> APSPIIKFPGDVAPKTDKELAVQYLNTFYGCPKESCNLFVLKDTLKKMQKFFGLPQTGDLDQNTIETMRKPRCGNPDVANYNFFPRKPKWDKNQITYRIIGYTPDLDPETVDDAFARAFQVWSDVTPLRFSRIHDGEADIMINFGRWEHGDGYPFDGKDGLLAHAFAPGTGVGGDSHFDDDELWTLGEGQVVRVKYGNADGEYCKFPFLFNGKEYNSCTDTGRSDGFLWCSTTYNFEKDGKYGFCPHEALFTMGGNAEGQPCKFPFRFQGTSYDSCTTEGRTDGYRWCGTTEDYDRDKKYGFCPETAMSTVGGNSEGAPCVFPFTFLGNKYESCTSAGRSDGKMWCATTANYDDDRKWGFCPDQGYSLFLVAAHAFGHAMGLEHSQDPGALMAPIYTYTKNFRLSQDDIKGIQELYGASPDIDLGTGPTPTLGPVTPEICKQDIVFDGIAQIRGEIFFFKDRFIWRTVTPRDKPMGPLLVATFWPELPEKIDAVYEAPQEEKAVFFAGNEYWIYSASTLERGYPKPLTSLGLPPDVQRVDAAFNWSKNKKTYIFAGDKFWRYNEVKKKMDPGFPKLIADAWNAIPDNLDAVVDLQGGGHSYFFKGAYYLKLENQSLKSVKFGSIKSD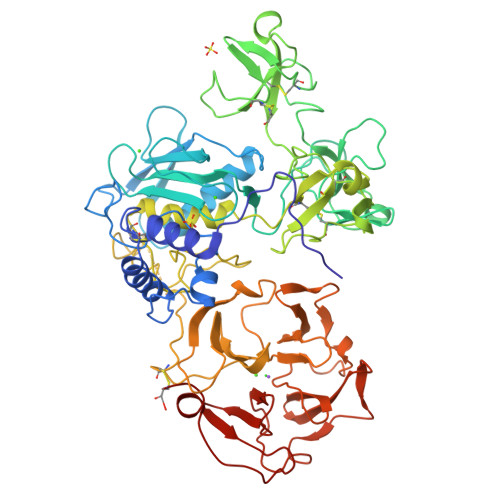WLGC> MKPKVFITRAIPENGINMLEEEFEVEVWEEEREIPREKLLEKVKDVDALVTMLSERIDQEVFENAPRLRIVANYAVGYDNIDVEEATRRGIYVTNTPDVLTNATADHAFALLLATARHVVKGDKFVRSGEWKRKGIAWHPKWFLGYELYGKTIGIVGFGRIGQAIARRAKGFNMRILYYSRTRKSQAEKELGAEYRPLEEVLKESDFVILAVPLTKETMYMINEERLKLMKPTAILVNIARGKVVDTKALIKALKEGWIAGAGLDVFEEEPYYNEELFSLDNVVLTPHIGSATFEAREAMAELVARNLIAFKRGEIPPTLVNKEVIKIRKPGFNEQ

Glyoxylate is a small and very reactive dicarboxylic acid molecule synthesized by most eukaryotes and prokaryotes. Considered as a toxic intermediate, this compound is metabolized by an unusual enzyme assigned to the D-2-hydroxy-acid dehydrogenase superfamily, glyoxylate reductase/hydroxypyruvate reductase (GRHPR). First, GRHPR is a dual activity enzyme. It catalyzes the reduction of glyoxylate into glycolate, which is either excreted or reconverted into glyoxylate (futile cycle) and the conversion of hydroxypyruvate into D-glycerate, a precursor supplying in the gluconeogenic pathway carbon.

For the first time, the determination of the PfuGRHPR structure reveals a ternary complex in the presence of glyoxylate. Indeed, the electron density showed unambiguously a smaller substrate compared to D-glycerate and was assigned to a glyoxylate molecule with full occupancy. Glyoxylate is located and oriented as D-glycerate in PyaGRHPR structure. Nonetheless, the absence of a hydroxymethyl moiety in the glyoxylate molecule (compared to D-glycerate) reduces the number of interaction between glyoxylate and the protein and induces shorter interactions distances. Two water molecules, separated by 2.69 Å, replace the single water molecule observed with D-glycerate. Unexpectedly, the catalytic Arg241, which is supposed to orient the substrate molecule12, is present in two conformations in the presence of glyoxylate. Additionally, the presence of glyoxylate led to the observation of a shift out the active site by 1.20 Å of Trp138, through a global movement of the protein main chain. A second glyoxylate molecule could be perfectly assigned to the observed electron density and was successfully refined with 50% occupancy. Detailed analysis of substrate interactions in the PfuGRHPR structure described in this paper shows the existence of a tunnel that controls the substrate trafficking. In particular, this tunnel is surrounded by Leu53, Trp138 and Arg241 and is large enough to accommodate a substrate molecule as illustrated by the presence of an additional glyoxylate molecule close to Trp138, providing a view of the substrate pathway.> MSKTESYCLEDALNDLFIPETTIETILKRLTIKKNIILQGPPGVGKTFVARRLAYLLTGEKAPQRVNMVQFHQSYSYEDFIQGYRPNGVGFRRKDGIFYN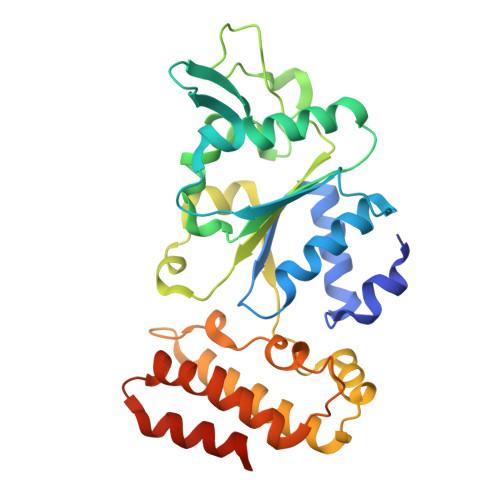FCQQAKEQPEKKYIFIIDEINRANLSKVFGEVMMLMEHDKRGENWSVPLTYSENDEERFYVPENVYIIGLMNTADRSLAVVDYALRRRFSFIDIEPGFDTPQFRNFLLNKKAEPSFVESLCQKMNELNQEISKEATILGKGFRIGHSYFCCGLEDGTSPDTQWLNEIVMTDIAPLLEEYFFDDPYKQQKWTNKLLGDSSGSHHHHHH> MNGRGFLIYNGGEKMKQKMIIYDTPAGPYPARVRIALAEKNMLSSVQFVRINLWKGEHKKPEFLAKNYSGTVPVLELDDGTLIAECTAITEYIDALDGTPTLTGKTPLEKGVIHMMNKRAEL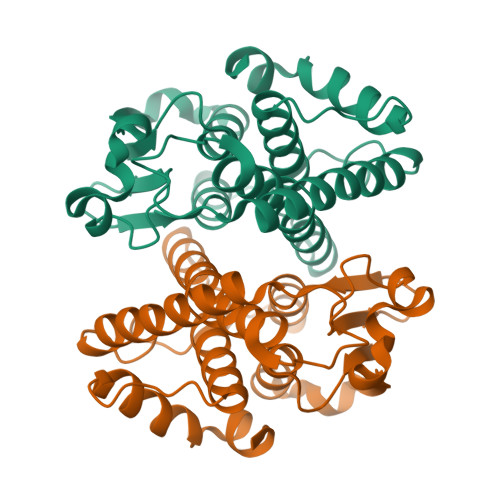ELLDPVSVYFHHATPGLGPEVELYQNKEWGLRQRDKALHGMHYFDTVLRERPYVAGDSFSMADITVIAGLIFAAIVKLQVPEECEALRAWYKRMQQRPSVKKLLEIRSKSS>SMGTKLKKSNNDITIFSENEYNEIVEMLRDYSNGDNLEFEVSFKNINYPNFMRITEHYINITPENKIESNNYLDISLIFPDKNVYRVSLFNQEQIGEFITKFSKASSNDISRYIVSLDPSDDIEIVYKNRGSGKLIGIDNWAITIKSTEEIPLVAGKSKISKPKITGSERIMYR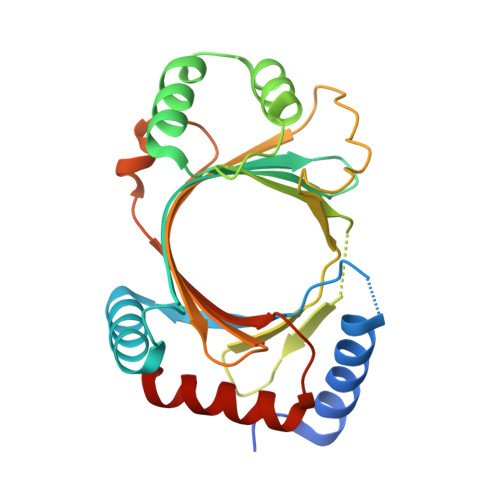YKTRYSFTINKNSRIDITDVKSSPIIWKLMTVPSNYELELELINKIDINTLESELLNVFMIIQD[2x]> GSHMSASC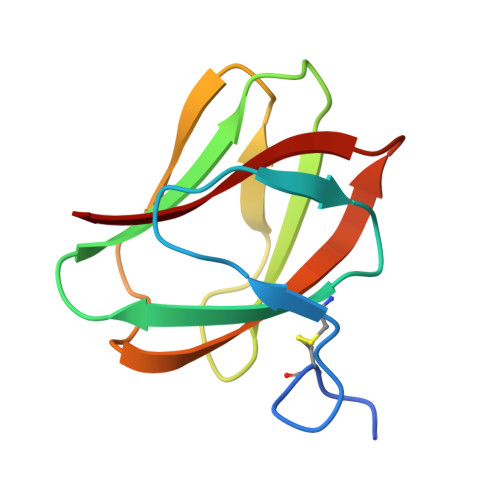GSGNFNKTAAKGVEFSAVAGDCIKYNKSSGTLQIGSWTGVASSYNITSGPQGITNTGNGWTTVANAANGDLYIKIVSASRSFNVKFDNW4-[(4-carboxybutanoyl)amino]benzene-1,2-dicarboxylic acid | C13 H13 N O7 | 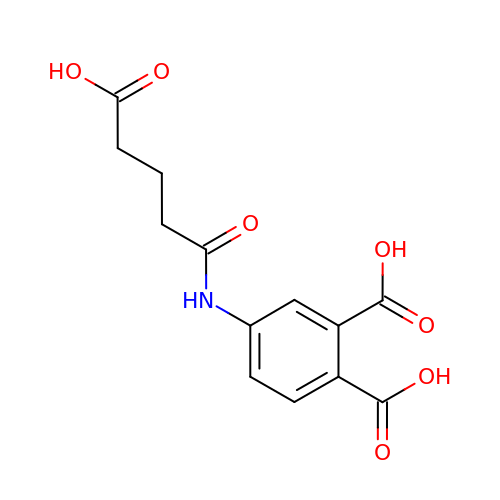XOVXZYVADZDQHJ-UHFFFAOYSA-N>[2x]MAESIRLAVAGVGNNISALFQGAELYRKMSAEGVAEADFPGIKRPRIGGIGVSDLTFVAAFDLHPNKVGVPFKDAVLAEPNNYPLLGVELPDPGFSVDAGLTEEDADPSSPAFRRIVERLRESKAEVLLYSLPTGLQWAAIAYARAALEAKVAFVNCTPELVARTPELLEEFEKAGVPLIGDDLASHLGTSVVHRALLGLLSERGLSLASSYQ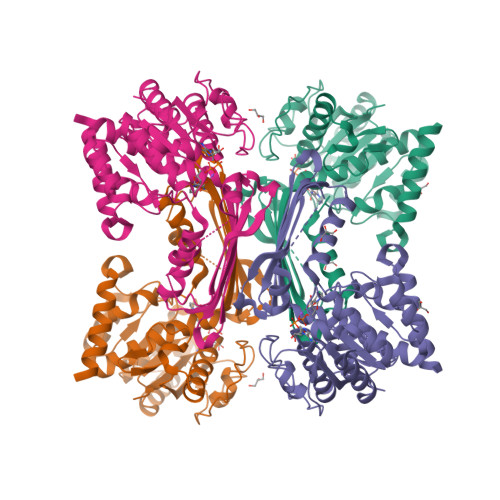LNLGGNEDFRNLRERGASKRQSKINALAQEGVDTSNVEVIPSAGYVAHLKDHKVAMLNIEGLGWAGTPVSIDLKLKVQDSSNAAGVIIDLIRIAAAARRVGFGGFSAAAVKVLKSPAGGHPSYTSEDVAEAYRQLDAVTEAMAEKDPNSSSVDKLAALEHHHHHH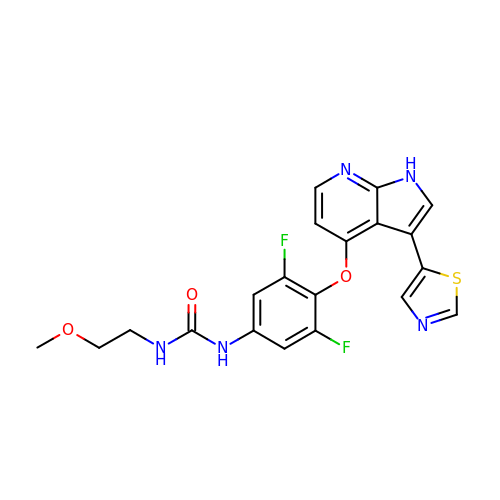1-[3,5-bis(fluoranyl)-4-[[3-(1,3-thiazol-5-yl)-1~{H}-pyrrolo[2,3-b]pyridin-4-yl]oxy]phenyl]-3-(2-methoxyethyl)urea | C20 H17 F2 N5 O3 S | GESKELIKUUWDIY-UHFFFAOYSA-N>GMAALLSQRQKRYQQFLAMKMTQVFDILFSLTRGQPYTETYLSSLIVDSLQDSNNPIGTKEASEILAGLQGILPM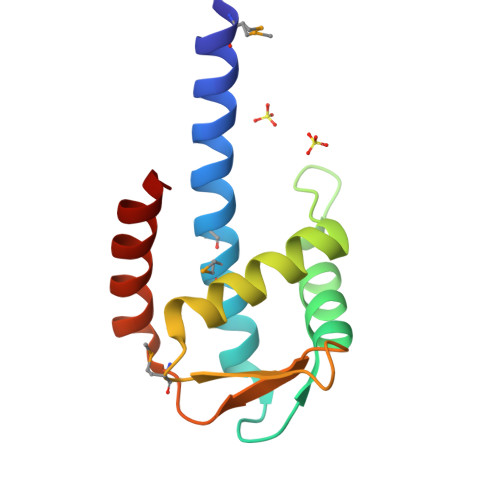DISVHQVDGGLKVYRWNSLDKNRFSKLLQIHKSKQQD[2x]>[2x]GAMAKIIHTADWHLGKILNG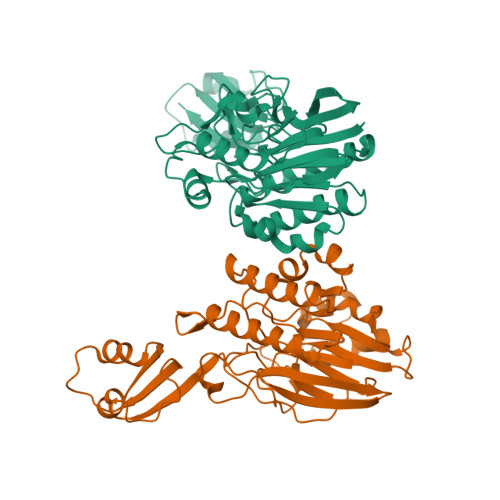KQLLEDQAYILDMFVEKMKEEEPDIIVIAGDLYDTTYPSKDAIMLLEQAIGKLNLELRIPIIMISGNHDGKERLNYGASWFEHNQLFIRTDFTSINSPIEINGVNFYTLPYATVSEMKHYFEDDTIETHQQGITRCIETIAPEIDEDAVNILISHLTVQGGKTSDSERPLTIGTVESVQKGVFDIFDYVMLGHLHHPFSIEDDKIKYSGSLLQYSFSEAGQAKGYRRLTINDGIINDVFIPLKPLRQLEIISGEYNDVINEKVHVKNKDNYLHFKLKNMSHITDPMMSLKQIYPNTLALTNET>MTATEELTFESTSRFAEVDVDGPLKLHYHEAGVGNDQTVVLLHGGGPGAASWTNFSRNIAVLARHFHVLAVDQPGYGHSDKRAEHGQFNRYAAMALKGLFDQLGLGRVPLVGNALGGGTAVRFALDYPARAGRLVLMGPGGLSINLFAPDPTEGVKRLSKFSVAPTRENLEAFLRVMVYDKNLITPELVDQRFALASTPESLTATRAMGKSFAGADFEAGMMWREVYRLRQPVLLIWGREDRVNPLDGALVALKTIPRAQLHVFGQCGHW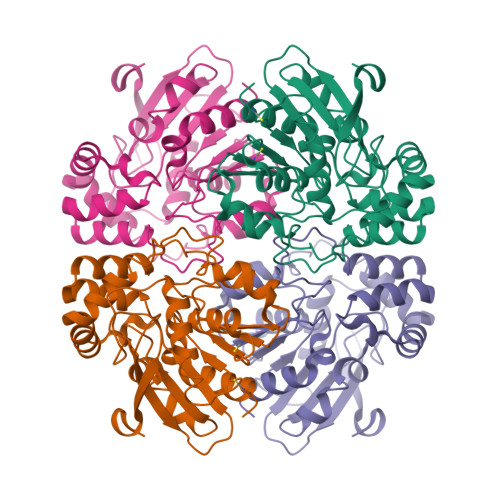VQVEKFDEFNKLTIEFLGGGR[2x]>[2x]MGIGIYSPGIWRIPHLEKFLAQPCQKLSLLRPVPQEVNAIAVWGHRPSAAKPVAIAKAAGKPVIRLEDGFVRSLDLGVNGEPPLSLVVDDCGIYYDASKPSALEKLVQDKAGNTALISQAREAMHTIVTGDMSKYNLAPAFVADESERTNIVLVVDQTFNCMSVTYGNAGPHEFAAMLEAAMAENPQAEIWVKVHPDVLEGKKTGYFADLRATQRVRLIAENVSPQSLLRHVSRVYVVTSQYGFEALLAGKPVTCFGQPWYASWGLTDDRHPQSALLSARRGSATLEELFAAAYLRYCRYIDPQTGEVSDLFTVLQWLQLQRRHHHHHH

KpsC is a dual-module glycosyltransferase (GT) essential for “group 2” capsular polysaccharide biosynthesis in Escherichia coli and other Gram-negative pathogens. Two separate GT modules in KpsC transfer 3-deoxy-β-d-manno-oct-2-ulosonic acid (β-Kdo) from cytidine-5′-monophospho-β-Kdo donor to a glycolipid acceptor. The N-terminal and C-terminal modules add alternating Kdo residues with β-(2→4) and β-(2→7) linkages, respectively, generating a conserved oligosaccharide core that is further glycosylated to produce diverse capsule structures. Based on the formation of covalent adducts with Kdo identified here by mass spectrometry and X-ray crystallography, we determined that catalytically important active site residues are conserved in WbbB and KpsC, suggesting a shared double-displacement mechanism.

Crystals of a ternary complex of KpsC-NEc were also generated using the D160C variant. While the structure of cysteine is less similar to aspartate than asparagine, the cysteine variant converts more fully to the adduct and was anticipated to be more stable on the multiweek timescale required for crystallization. The D160C variant was expressed in E. coli BL21 (DE3) and then crystallized in the presence of 1 mM CMP and 5 mM acceptor 2, a β-Kdo-(2→7)-β-Kdo disaccharide. The structure of this complex was determined at 1.20 Å resolution; notably, this appears to be among the highest resolution structures currently determined for a GT. The resulting map revealed highly detailed density for the Cys160–Kdo adduct and for acceptor molecules in both copies of the active site present in the asymmetric unit. Chain A, which contains CMP, the Kdo-adduct, and the acceptor, is the focus of the discussion below. Cys160 Cα is shifted roughly 1 Å into the catalytic pocket to compensate for its shorter side chain (compared to aspartate or asparagine), and the anomeric carbon (C2) is shifted 0.5 Å towards Asp/Asn/Cys160. One noticeable difference is that the C1 carboxylate rotates ∼90° and hydrogen bonds with the guanidinium group of Arg45. The acceptor disaccharide interacts almost exclusively with residues from the N-terminal α/β domain. The C1 carboxylate group of Kdo-A1 is hydrogen bonded to Lys202 (the only directly interacting residue from outside the N-terminal α/β domain), as well as to Kdo-A1 O8.>[2x]QSEPELKLESVVIVSRHGVRAPTKATQL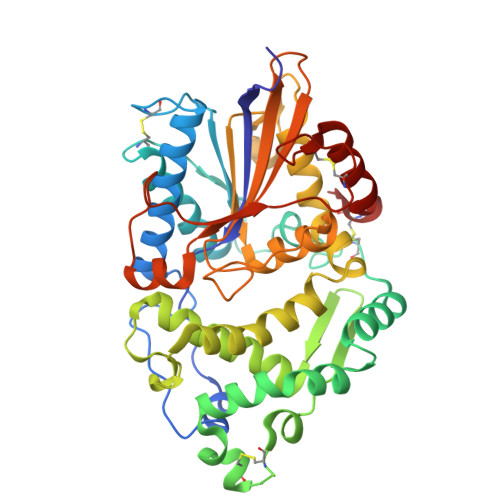MQDVTPDAWPTWPVKLGWLTPRGGELIAYLGHYQRQRLVADGLLAKKGCPQSGQVAIIADVDERTRKTGEAFAAGLAPDCAITVHTQADTSSPDPLFNPLKTGVCQLDNANVTDAILSRAGGSIADFTGHRQTAFRELERVLNFPQSNLCLKREKQDESCSLTQALPSELKVSADNVSLTGAVSLASMLTEIFLLQQAQGMPEPGWGRITDSHQWNTLLSLHNAQFYLLQRTPEVARSRATPLLDLIKTALTPHPPQKQAYGVTLPTSVLFIAGHDTNLANLGGALELNWTLPGQPDNTPPGGELVFERWRRLSDNSQWIQVSLVFQTLQQMRDKTPLSLNTPPGEVKLTLAGCEERNAQGMCSLAGFTQIVNEARIPACSL> PNSLEAQIRQAMKTGSTLTIEFDQALNQKSPGTLNVFLHPANGGVRIDLDSGNQGEPAKILWLPWKQGELQTLQPGSISTVDMLFFTYYLSGCKVFAGDGGPVWHIDAPVEANQFWRRMSSDEWMEDWEVGTDRQVAYLHRAGQSDSLWNLSAYLEGAAPSTYGRDNLGQAVVGGIVTGRQQ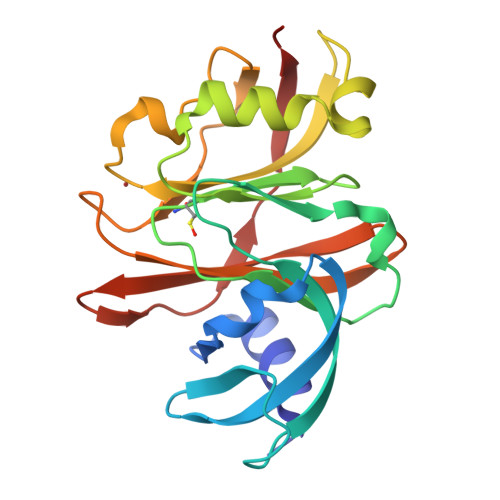MSLYQYATTSSGSSAWSPLTYTLQQRKQ> FPTIPLSRLADNAWLRADRLNQLAFDTYQEFEEAYIPKEQIHSFW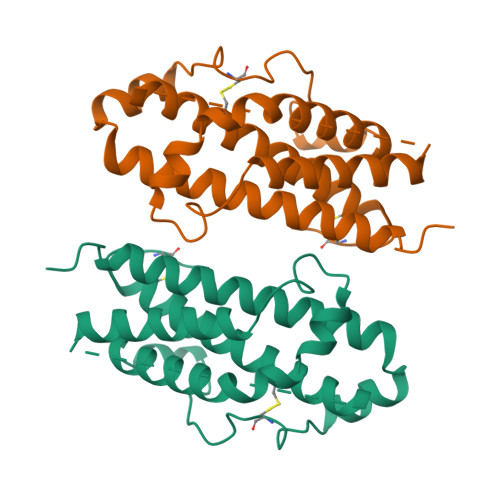WNPQTSLCPSESIPTPSNKEETQQKSNLELLRISLLLIQSWLEPVQFLRSVFANSLVYGASDSNVYDLLKDLEEGIQTLMGRLEDGSPRTGQIFKQTYSKFDTNSHNDDALLKNYGLLYCFNKDMSKVSTYLRTVQCRSVEGSCGF> G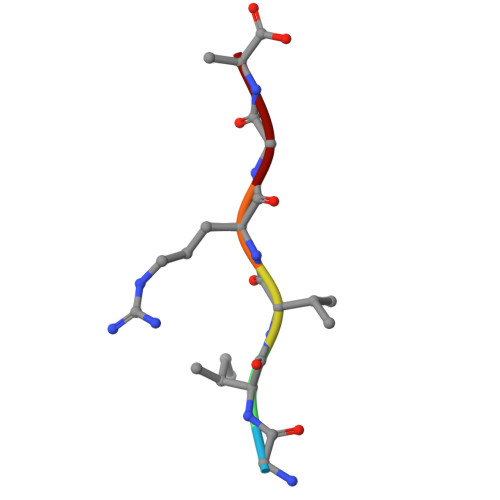IVRGA> QTIQPGTGYNNGY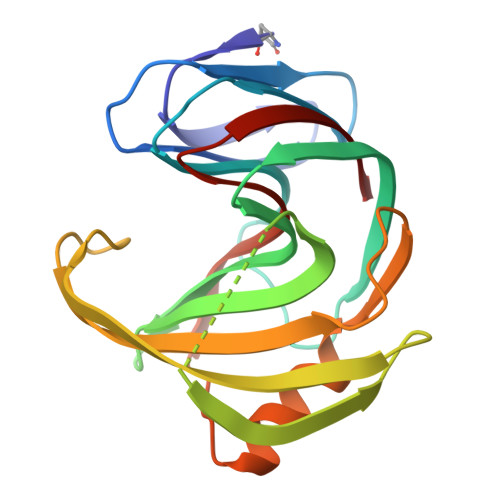FYSYWNDGHGGVTYTNGPGGQFSVNWSNSGNFVGGKGWQPGTKNKVINFSGSYNPNGNSYLSVYGWSRNPLIEYYIVENFGTYNPSTGATKLGEVTSDGSVYDIYRTQRVNQPSIIGTATFYQYWSVRRNHRSSGSVNTANHFNAWAQQGLTLGTMDYQIVAVEGYFSSGSASITVS>[4x]MVKVDLESKRYGEKLKEVFLMLDNNVVECIKEITESSRNGKLVFFVGAGVSTLSDYPQWWRLVDKYHEELYGSPKKGNYSSDEYLRIPQIFYNVKGEMAFDGILKDFFQVDKPTNPIHDKILAMNPAHVITTNYDNLIDTACWKRGKYFSVISAEEDVANATSSRYLLKVHGDFRKGFKGENVVLKEDDYLNYDQNYPLISNLMKTIIATHTIVFIGYGLGDYNINMLLNWVRKLQKDSFHKPFFIRTDPSPIENETLIYYENKGLRIIDAASLIDSNEYDYLERYSAVMDLLIESQENKFITKDDEVIDYIYGKISPLFALQYIRKIDLKHVFEYDYHFEVNGTVVRHKNKGFGYMERFFELKESCDERSKLSKKQYERFNALFNFFEKNGVICMAKDAGTLNTSIEINSLAYHGKYDVMKKFIEEQSVSIEDDYKKAFFLACLGRWEESYDLYSNIILNSIDESNGCVYYLSQINRYRIYQSITQAVTQFNGLGLLTFGRHYKPFTDEFLARIEREMTNFNIDDLFNGMPFEFQKKYKILEFLSDNQFLYDDTVKLFELTNKVRSEMSEGSYSFGMSSDIV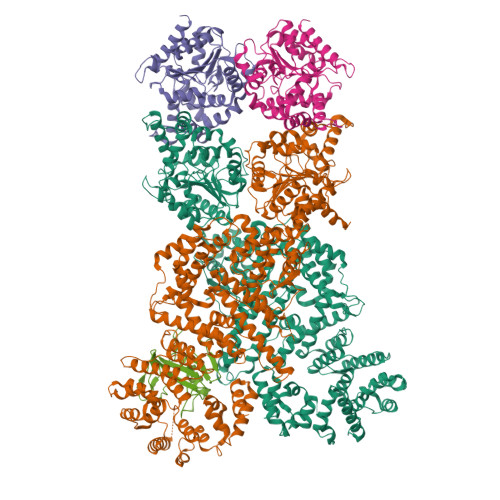VLLRLYDNLRFLYENCLWSVSFHEFHQYIRNSMSLLIEKAEYERTRDIDELGFSFFGKKSGFFMEYYDFVNISRHFKIDDIKNLERSCSIDKIRFGEQEKIEEYLVGIAEEITKQFSANGMNVVFYTQFISEAKAALYFAKYVKLSEEGLGKIVKALLFYFPERDLDIGKRYVWLERLTKCNELPKSIISIIDDFLVLQAEKHIDQNYSEVSSNGLYSRDYGALIKHFEKNFISKRLSEITLCLTQDKQKQIDFLFKLLPLLSTNAKSHLLSFKSVENINDLMNGIRIGLIDEFTPEHEELIIEYLETRKVNYIVEKEKGIQTFSSNDYMSTFGIWYFLEEINNSKMEEFIGMDDQYDFFVDPENFDYKKFIPSWLKNYNDKLLGKIAGNKHMKHHVIEVLKERVKNSNDKRYLEILMNYFI;> MIEIFKDTGATHDLVYHSKINTFVWDVEFDIVLSDSKELNKCYFVKCFNPYRINGKCDFAVSSIDIFSEGKRLLIENEFNFKITKAVHVATSKDVTEIVLHLSERISSPFPIVKEVVYLD> SNATGLGELKISDTICAQNAVEALPALSVDEPTVTMTFQVNTSPFAGKEGKFVTSRNILERLEKELVHNVALRVEQTDDPDKFRVSGRGELHLSILIENMRREGFELAVSRPEVIIKEEDGQLMEPFETVTIDVM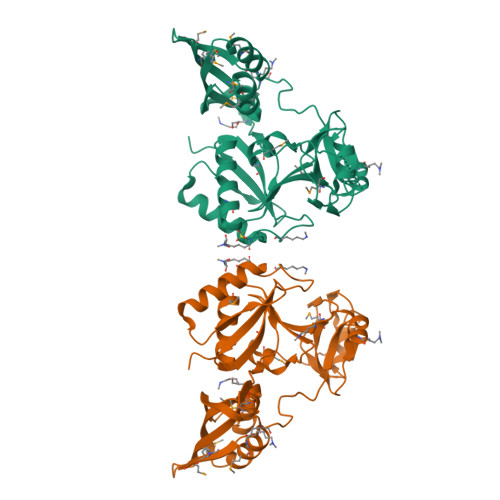EEHQGGIMENIGLRKGELKDMAPDGKGRVRMDFIMPSRGLIGFQTEFMTLTSGSGLLYHTFDHYGPHKGGNIGQRVNGVLIANAAGKALTNALFNLQERGRLFIGHGVEVYEGMVIGIHSRDNDLTVNALKGKQLTNVRASGTDDAQVLTPPIVMTLEQALEFIDDDELVEVTPESIRIRKKFLTESDRKRASRSAK>[2x]MSEPMMWLLVRGVWETLAMTFVSGFFGFVIGLPVGVLLYVTRPGQIIANAKLYRTVSAIVNIFRSIPFIILLVWMIPFTRVIVGTSIGLQAAIVPLTVGAAPFIARMVENALLEIPTGLIEASRAMGATPMQIVRKVLLPEALPGLVNAATITLITLVGYSAMGGAVGAGGLGQIGYQYGYIGYNATVMNTVLVLLVILV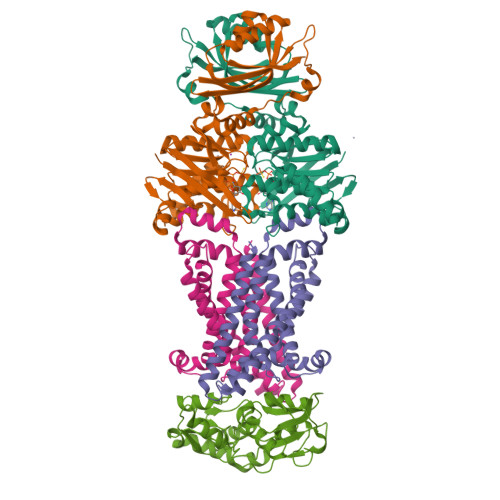YLIQFAGDRIVRAVT;>[2x]HMIKLSNITKVFHQGTRTIQALNNVSLHVPAGQIYGVIGASGAGKSTLIRCVNLLERPTEGSVLVDGQELTTLSESELTKARRQIGMIFQHFNLLSSRTVFGNVALPLELDNTPKDEVKRRVTELLSLVGLGDKHDSYPSNLSGGQKQRVAIARALASNPKVLLCDQATSALDPATTRSILELLKDINRRLGLTILLITHEMDVVKRICDCVAVISNGELIEQDTVSEVFSHPKTPLAQKFIQSTLHLDIPEDYQERLQAEPFTDCVPMLRLEFTGQSVDAPLLSETARRFNVNNAIISAQMDYAGGVKFGIMLTEMHGTQQDTQAAIAWLQEHHVKVEVLGYV;> KVGVIVGAEQQVAEVAQKVAKDKYGLDVELVTFNDYVLPNEALSKGDIDANAFQHKPYLDQQLKDRGYKLVAVGNTFVYPIAGYSKKIKSLDELQDGSQVAVPNDPTNLGRSLLLLQKVGLIKLKDGVGLLPTVLDVVENPKNLKIVELEAPQLPRSLDDAQIALAVINTTYASQIGLTPAKDGIFVEDKESPYVALIVTREDNKDAENVKKFVQAYQSDEVYEAA>GVNPRGLGPLQIWQTDFTLEPRMAPRSWLAVTVDTASSAIVVTQHGRVTSVAVQHHWATAIAVLGRPKAIKTDNGSCFTSKSTREWLARWGIAHTTGIPGNSQGQAMVERANRLLKDRIRVLAEGDGFMKRIPTSKQGELLAKAMYALNHKERGENTKTPIQKHWRPTVLTEGPPVKIRIE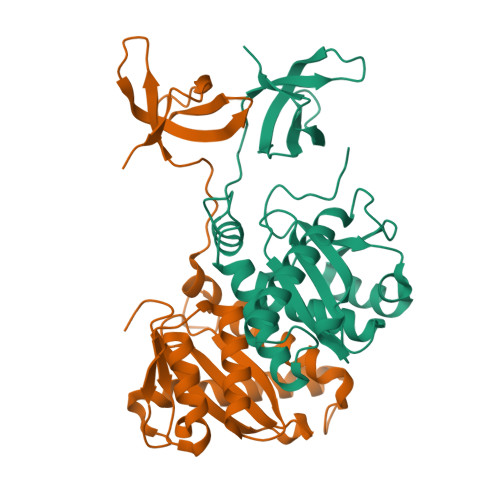TGEWEKGWNVLVWGRGYAAVKNRDTDKVIWVPSRKVKPDITQKDEVTKKDEASPLFA[4x]> MTSKTKNIDDIPPEIKEEMIQLYHDLPGIENEYKLIDKIGEGTFSSVYKAKDITGKITKKFASHFWNYGSNYVALKKIYVTSSPQRIYNELNLLYIMTGSSRVAPLCDAKRVRDQVIAVLPYYPHEEFRTFYRDLPIKGIKKYIWELLRALKFVHSKGIIHRDIKPTNFLFNLELGRGVLVDFGLAEAQMDYKSMISSQNDYDNYANTNHDGGYSMRNHEQFCPCIMRNQYSPNSHN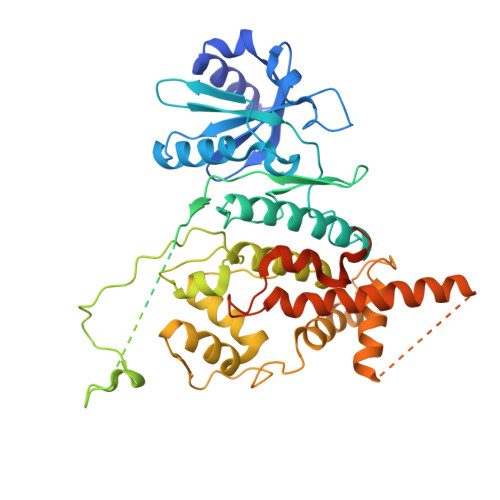QTPPMVTIQNGKVVHLNNVNGVDLTKGYPKNETRRIKRANRAGTRGFRAPEVLMKCGAQSTKIDIWSVGVILLSLLGRRFPMFQSLDDADSLLELCTIFGWKELRKCAALHGLGFEASGLIWDKPNGYSNGLKEFVYDLLNKECTIGTFPEYSVAFETFGFLQQELHDRMSIEPQLPDPKTNMDAVDAYELKKYQEEIWSDHYWCFQVLEQCFEMDPQKRSSAEDLLKTPFFNELNENTYLLDGESTDEDDVVSSSEADLLDKDVLLISE>[2x]SIGLALLLLLLALLFWLYIVMSNWTGGALLVLYSFALMLIIIILII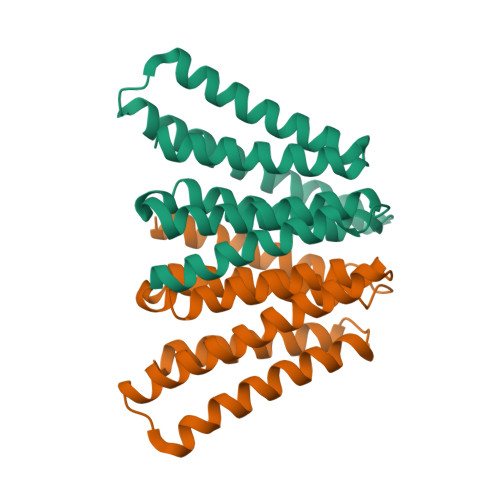FIFRRDLLCPLGGLGLLLLMITLLLIALWNLHGQALYLGIVLFIFGCLLVLGLWIYFLEILWRLGATIWQLLAFILAFFLAIILLIIALYLQQNWWTLLVDLLWLLLFMAILIWMY>[2x]MAAEDFLTIFLDDDESWNETLNMSGYDYSGNFSLEVSVCEMTTVVPYTWNVGILSLIFLINVLGNGLVTYIFCKHRSRAGAIDILLLGICLNSLCLSISLLAEVLMFLFPNIISTGLCRLEIFFYYLYVYLDIFSVVCVSLVRYLLVAYSTRSWPKKQSLGWVLTSAAWLIALVLSGDACRHRSRVVDPVSKQAMCYENAGNMTADWRLHVRTVSVTAGFLLPLALLILFYALTWCVVRRTKLQARRKVRGVIVAVVVLFFVFCFPYHVLNLLDTLLRRRWIRDSCYTRGLINVGLAVTSLLQALYSAVVPLIYSCLGSLFRQRMYGLFQSLRQSFMSGADYKDDDDKGRPLEVLFQGPHHHHHHHHHH

Kaposi’s Sarcoma-associated Herpesvirus encodes ORF74, a viral G protein-coupled receptor homologous to CXCR2, which plays a crucial role in Kaposi’s Sarcoma development through its high basal signaling activity. ORF74 was identified as a homolog of the chemokine receptor CXCR2, which is a member of the class A GPCR subfamily. ORF74 has been shown to have robust and high basal activity for multiple signaling pathways. In this study, we present cryoEM structures of ORF74 in ligand-free, BRIL-fused ligand-free, and CXCL1 & Gitrimer(Gαi/Gβ1/Gγ2)-bound states, providing an inactive-active pair of structures of a vGPCR, allowing comparisons and insights into the likely conformational transitions.

To obtain the inactive structure of ORF74, we expressed and purified ORF74 without the agonist CXCL1. We optimized the sample for cryoEM by reconstituting the detergent-purified apo-ORF74 in nanodiscs (first panel). CryoEM analysis revealed homodimer formation in the nanodiscs, enabling structure determination at 2.9 Å resolution despite ORF74’s small size (~38 kDa). Unexpectedly, atomic modeling showed an antiparallel orientation of the two protomers, an uncommon feature among GPCRs, likely induced during purification. Nevertheless, the apo-ORF74 model from the antiparallel dimer showed a strong structural fit to the BRIL-fused ORF74 map, while the CXCL1 & Gitrimer-bound ORF74 differed significantly. This suggests that the apo-ORF74 structure represents a bona fide inactive conformation. To further investigate whether the apo conformation adopts an inactive form, we compared the apo protomer model of ORF74 with the known inactive conformation of CXCR240. An RMSD of 1.7 Å from their superposition suggested similarities between these two structures including the positioning of the ECL2, 7 TMs, and ICL3. Notably, in both structures, ICL3 occupies a position that would sterically clash with the incoming Gαi/α5-helix of the Gitrimer in the active conformation. Structural analysis of inactive ORF74 revealed a segmented TM6 helix, composed of distinct TM6a and TM6b regions.3-DIPHENOL-6-NITRO-3H-BENZO[DE]ISOCHROMEN-1-ONE | C24 H15 N O6 | 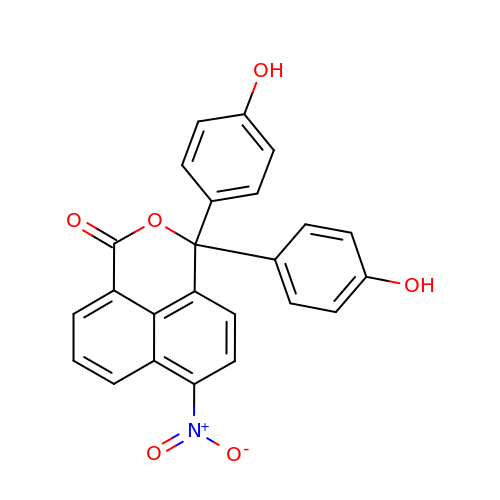FLWABCQDXUKNQY-UHFFFAOYSA-N> EEWE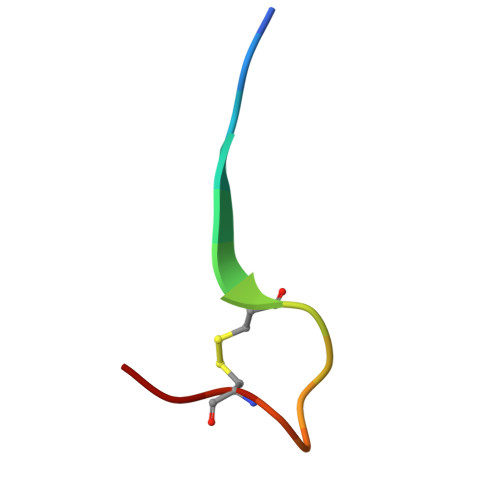VLCWTWETCER>MAMTVTEVDLPPIYCPLE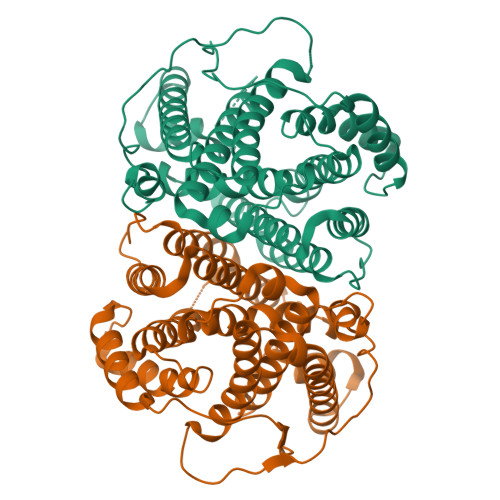SAIHPRVHEVEKRAVEWIRRSGMCASEEERAWVIATHSADFFARFAPTAADEDRLLATSLWVYWGFAFDDHRCDNGPLSTRPAQFNALAGRVQRALEAPSAEDNGDRFVPALQDIARRFRSFGTPTQVRRFVHAHRAYLSGVAWQIGNQARGHMPGLDDYLAMRLLSAGGEPTFAMLEIATGAEVPDREMHRPAVRALTEMAIMVAALDNDRHSLRKELSRGHTDQNIYSVLMHHRGMSLQEAVEEATKLRDRILLRFLELHDRVRPGAGAELSTYLQGLRHGIRGNAEWGLRVPRYLSLGRVPDPMEDAPLTWAESPSDSSPSPLPGAPSIAWWWDDALLGA[2x]> SEPYQIDIRRATNTDAW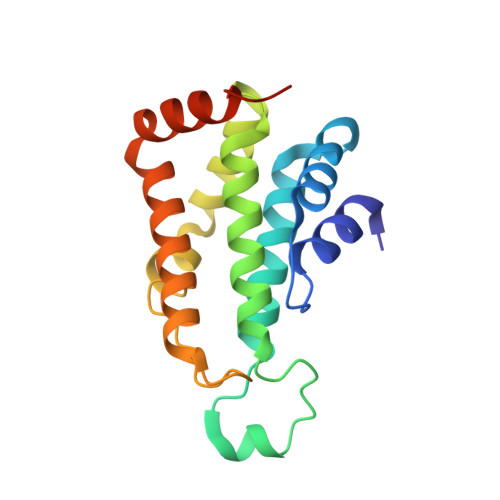GPTPKHLAKVLRNRYQVPLYLMTEYTLKRLVDHIATRPKNLYEKARKDYVNYGSEWRVVLKCLVVIEFLLLNVDTGDELNQIRSCLLTHKHILTREIAQFKVKFSNDGKMEIHERGIRKKGELILQYLEDSQFLKKERAKNKKNALEHHHHHH> GPGGSGGMKPQIRNMVEPMDPRTFVSNFNNRPILSGLDTVWLCCEVKTKDPSGPPLDAKIFQGKVYPKAKYHPEMRFLRWFHKWRQLHHDQEYKVTWYVSWSPCTRCANSVATFLAKDPKVTLTIFVARLYYFWKPDYQQALRILAEAGATMKIMNYNEFQDCWNKFVDGRGKPFKPWNNLPKHYTLLQATLGELLRHLMDPGTFTSNFNNKPWVSGQHETYLCYKVERLHNDTWVPLNQHRGFLRNQAPNIHGFPKGRHAALCFLDLIPFWKLDGQQYRVTCFTSWSPCFSCAQEMAKFISNNEHVSLCIFAARIYDDQGRYQEGLRTLHRDGAKIAMMNYSE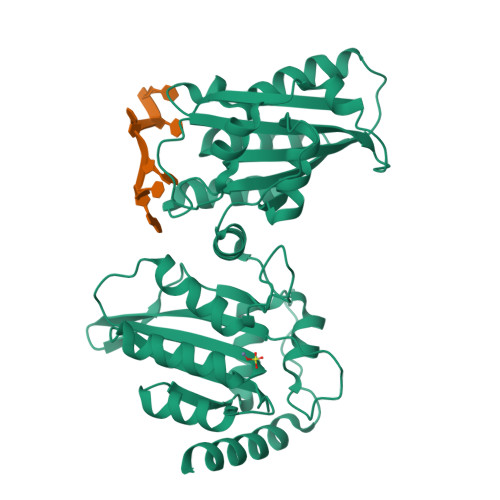FEYCWDTFVDRQGRPFQPWDGLDEHSQALSGRLRAILQNQGN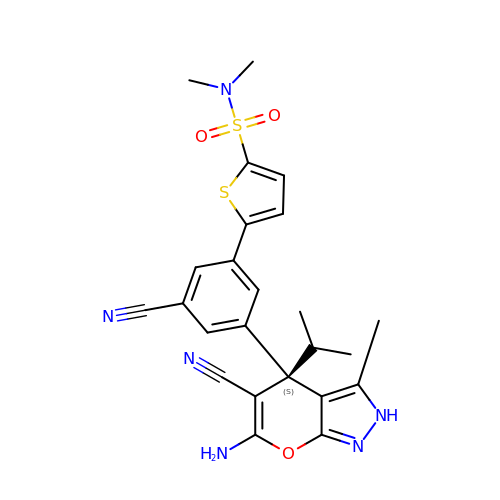5-[3-[(4~{S})-6-azanyl-5-cyano-3-methyl-4-propan-2-yl-2~{H}-pyrano[2,3-c]pyrazol-4-yl]-5-cyano-phenyl]-~{N},~{N}-dimethyl-thiophene-2-sulfonamide | C24 H24 N6 O3 S2 | KSCQEXGCEZGBHT-DEOSSOPVSA-N>GSFTMADLDDIKDGKDFRTDQPQKNIPFTLKGCGALDWGMQSRLSRIFNPKTGKTVMLAFDHGYFQGPTTGLERIDINIAPLFEHADVLMCTRGILRSVVPPATNRPVVLRASGANSILAELSNEAVALSMDDAVRLNSCAVAAQVYIGSEYEHQSIKNIIQLVDAGMKVGMPTMAVTGVGKDMVRDQRYFSLATRIAAEMGAQIIKTYYVEKGFERIVAGCPVPIVIAGGKKLPEREALEMCWQAIDQGASGVDMGRNIFQSDHPVAMMKAVQAVVHHNETADRAYELYLSEKQ[20x]

While sequence analysis suggests that LsrF will function as a class I aldolase and genetic data suggests LsrF is involved in P-AI-2 processing, the details of the role LsrF plays in processing P-AI-2 are not known. To begin addressing this question, we have determined the crystal structure of LsrF, alone and in complex with the P-AI-2 analogues ribose-5-phosphate and ribulose-5-phosphate. LsrF crystallizes as a decamer with each monomer having an (αβ)8-barrel fold, a ubiquitous fold commonly seen in proteins catalyzing aldolase reactions. The LsrF oligmer has a disk-like structure, with two rings of five monomers stacked on top of each other giving rise to a decamer with D5 symmetry.

To identify the catalytic site of LsrF, we determined the structure of the protein in complex with two P-AI-2 analogues: ribose-5-phosphate (R5P) and ribulose-5-phosphate (5RP). In both structures, the ligand electron density allowed definitive placement of the phosphate group and illustrated the general path of the carbon chain, but was of insufficient quality for unambiguous placement of all ligand atoms. As an independent confirmation of placement of the phosphate, the LigandFit module of PHENIX was used as an automated means for placing the ligands. The automated procedure positioned the phosphates in the same location as was modeled manually. R5P and 5RP bind LsrF in the same location, near the entrance to the (αβ)8-barrel with the phosphate group oriented towards the coils following β7 and β8. The phosphate is located near the positively charged side chain of Arg254 and is positioned to form hydrogen bonds with the side chain of His58, the side chain and main chain of Arg254, and the main chain of three glycine residues: 226, 227, and 253 (in all cases with N or NH groups). The ligand then extends across the center of the (αβ)8-barrel, away from strands 7 and 8, in a largely polar environment. In particular, Lys203 is adjacent to the ligand; this residue has potential significance for the mechanism, as equivalently positioned lysines are responsible for Schiff base formation in other aldolases (below). No large conformational changes were observed upon ligand binding, though there were small movements in a few binding site residues, most notably Asp251 and Met252 (with α-carbons shifting by 0.5–2.0 Å). The P-AI-2 analogues ribose-5-phosphate and ribulose-5-phosphate bind to LsrF in the same general position that other aldolases bind phosphorylated substrates (e.g. E. coli DERA and FBPA, T. tenax FBPA and M. jannaschii ADH synthase), suggesting that the canonical aldolase active site is conserved in LsrF.>[2x]MGHHHHHHHHHHSSGHIEGRHMMRAIWTGSIAFGLVNVPVKVYSATADHDIRFHQVHAKDNGRIRYKRVCEACGEVVDYRDLARAYESGDGQ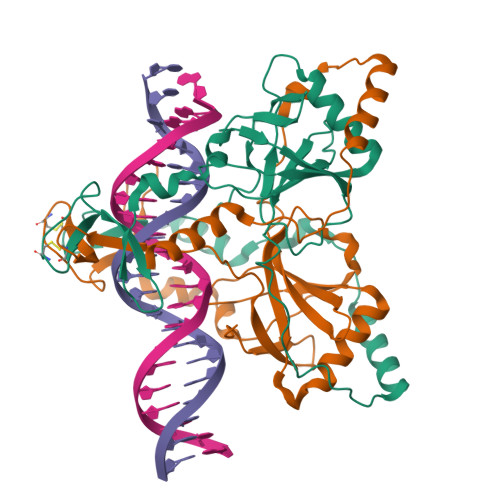MVAITDDDIASLPEERSREIEVLEFVPAADVDPMMFDRSYFLEPDSKSSKSYVLLAKTLAETDRMAIVHFTLRNKTRLAALRVKDFGKREVMMVHTLLWPDEIRDPDFPVLDQKVEIKPAELKMAGQVVDSMADDFNPDRYHDTYQEQLQELIDTKLEGGQAFTAEDQPRLLDEPEDVSDLLAKLEASVKARSKANSNVPTPP Channelrhodopsins, light-gated cation channels, enable precise control of neural cell depolarization or hyperpolarization with light in the field of optogenetics. The first crystal structure of a channelrhodopsin has been solved for a chimera between Channelrhodopsin-1 and Channelrhodopsin-2 from C. reinhardtii commonly known as C1C2.4 This chimera with transmembrane helices (TM) 1–5 from ChR1 and 6–7 from ChR2 is more stable in detergent than the parental ChRs and provided the first invaluable insight into the overall architecture of the central ion conducting core. It shares the prototypical seven-transmembrane helical fold of microbial ion pumps and human G protein-coupled receptors. A first constriction of the putative channel, called the central gate which is composed of residues Glu129, Asn297 and Ser102, is found close to the retinal Schiff base and its counterion residues Glu162 and Asp292 (Channelrhodopsin-2 numbering can be obtained by subtracting 39 from the C1C2 residue numbers).

For our room temperature analysis of light-induced conformational changes in C1C2 we purified recombinant C1C2 from insect cells and grew crystals in lipidic mesophases following established conditions and subjected them to serial synchrotron crystallography at the Swiss Light Source, where they diffracted with anisotropic resolution up to 2.6 Å. To elucidate the conformational changes required to fully open the channel, we performed atomistic molecular dynamics (MD) simulations starting from the light-activated structure. As a further control, we performed the same simulations starting from the dark state structure. In both the dark-state and M390b protonation state simulations, the channel remained closed with no K+ permeation events. Even though the central gate and extracellular vestibule in the light-activated structure were more open compared to the dark-state structure, the changes were not sufficient to allow K+ permeation.

> STGSDATVPVATQDGPDYVFHRAHERMLFQTSYTLENNGSVICIPNNGQCFCLAWLKSNGTNAEKLAANILQWITFALSALCLMFYGYQTWKSTCGWEEIYVATIEMIKFIIEYFHEFDEPAVIYSSNGNKTVWLRYAEWLLTCPVILIHLSNLTGLANDYNKRTMGLLVSDIGTIVWGTTAALSKGYVRVIFFLMGLCYGIYTFFNAAKVYIEAYHTVPKGRCRQVVTGMAWLFFVSWGMFPILFILGPEGFGVLSVYGSTVGHTIIDLMSKNCWGLLGHYLRVLIHEHILIHGDIRKTTKLNIGGTEIEVETLVEDEAEAGAVSSEDLYFQ>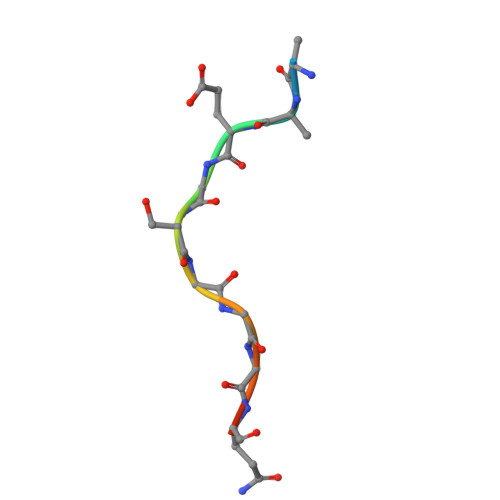 QEEEGSGGGQGG>[2x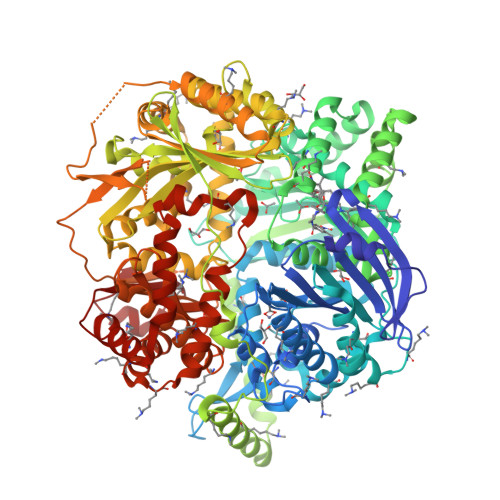]MHHHHHHAAACERALQYKLGDKIHGFTVNQVTSVPELFLTAVKLTHDDTGARYLHLAREDTNNLFSVQFRTTPMDSTGVPHILQHTVLCGSQKYPCRDPFFKMLNRSLSTFMNAFTASDYTLYPFSTQNPKDFQNLLSVYLDATFFPCLRELDFWQEGWRLEHENPSDPQTPLVFKGVVFNEMKGAFTDNERIFSQHLQNRLLPDHTYSVVSGGDPLCIPELTWEQLKQFHATHYHPSNARFFTYGNFPLEQHLKQIHEEALSKFQKIEPSTVVPAQTPWDKPREFQITCGPDSFATDPSKQTTVSVSFLLPDITDTFEAFTLSLLSSLLTSGPNSPFYKALIESGLGTDFSPDVGYNGYTREAYFSVGLQGIVEKDIETVRSLIDRTIDEVVEKGFEDDRIEALLHKIEIQMKHQSTSFGLMLTSYIASCWNHDGDPVELLKLGNQLAKFRQCLQENPKFLQEKVKQYFKNNQHKLTLSMRPDDKYHEKQAQVEATKLKQKVEALSPGDRQQIYEKGLELRSQQSKPQDASCLPALKVSDIEPTIPVTELDVVLTAGDIPVQYCAQPTNGMVYFRAFSSLNTLPEELRPYVPLFCSVLTKLGCGLLDYREQAQQIELKTGGMSASPHVLPDDSHMDTYEQGVLFSSLCLDRNLPDMMQLWSEIFNNPCFEEEEHFKVLVKMTAQELANGIPDSGHLYASIRAGRTLTPAGDLQETFSGMDQVRLMKRIAEMTDIKPILRKLPRIKKHLLNGDNMRCSVNATPQQMPQTEKAVEDFLRSIGRSKKERRPVRPHTVEKPVPSSSGGDAHVPHGSQVIRKLVMEPTFKPWQMKTHFLMPFPVNYVGECIRTVPYTDPDHASLKILARLMTAKFLHTEIREKGGAYGGGAKLSHNGIFTLYSYRDPNTIETLQSFGKAVDWAKSGKFTQQDIDEAKLSVFSTVDAPVAPSDKGMDHFLYGLSDEMKQAHREQLFAVSHDKLLAVSDRYLGTGKSTHGLAILGPENPKIAKDPSWIIR>GSSGSSGMASSCAVQVKLELGHRAQVRKKPTVEGFTHDWMVFVRGPEHSNIQHFVEKVVFHLHESFPRPKRVCKDPPYKVEESGYAGFILPIEVYFKNKEEPRKVRFDYDLFLHLEGHPPVNHLRCEKL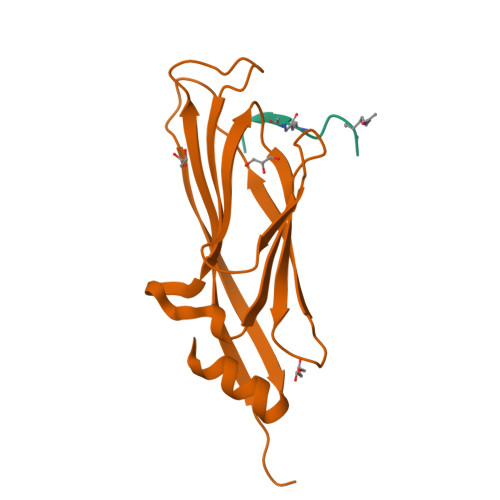TFNNPTEDFRRKLLKA[2x];> SGRGKGGKGLGK>[4x]MGHHHHHHQQIMKGNFSSFMQKEIFEQPESVVNTMRGRVNFDDYTVNLGGLKDHIKEI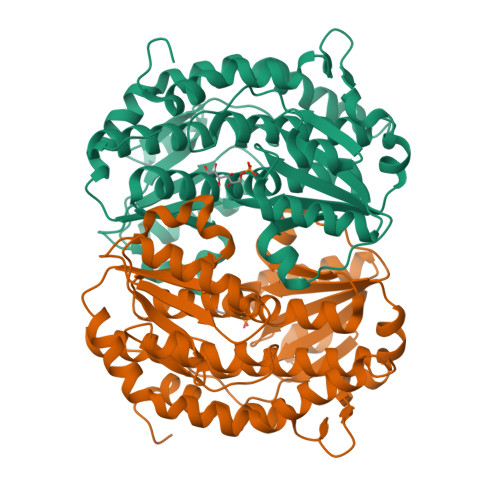QRCRRLILIACGTSYHAGVATRQVLEELTELPVMVELASDFLDRNTPVFRDDVCFFLSQSGETADTLMGLRYCKERGALTVGITNTVGSSISRETDCGVHINAGPEIGVASTKAYTSQFVSLVMFALMMCDDRISMQERRKEIMLGLKRLPDLIKEVLSMDDEIQKLATELYHQKSVLIMGRGYHYATCLEGALKIKEITYMHSEGILAGELKHGPLALVDKLMPVIMIIMRDHTYAKCQNALQQVVARQGRPVVICDKEDTETIKNTKRTIKVPHSVDCLQGILSVIPLQLLAFHLAVLRGYDVDFPRNLAKSVTVE> MGAVERLA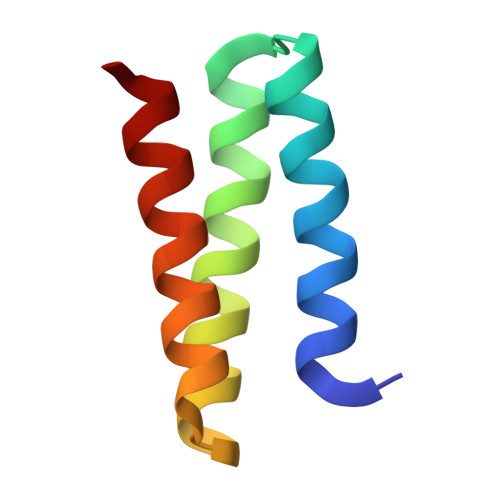EKAYELLKLVKEAAPLEEVKELADEIIAEAEAALAEKPSVELKVILELAKELLEEAEK> MADNSDDYSYD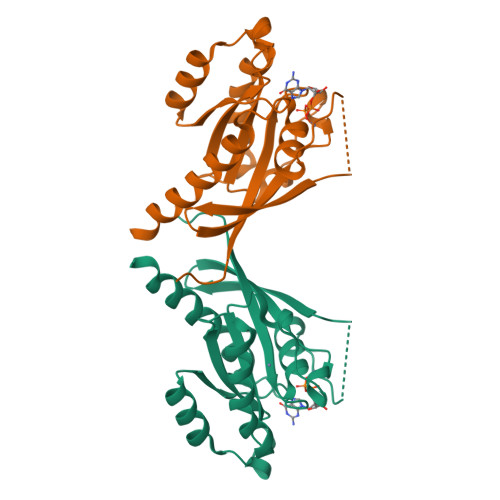YEYLYKIVLIGDSGVGKSNLLSRFTRDEFNLESRSTIGVEFATRTLEIDGKRVKAQIWDTAGQERYRAITSAYYRGAVGALIVYDIAKTESYESVSRWLKELKEHADANIIIELVGNKSDLDHLRAVPTEEAKNFAMENNLLFTEASALSSDNVDLSFHQLLKNIYEMISKHQLENNDSKQTNTAGGPTISLTPAPQEKKNKNNGXLLLRH> DFQSESYKDAYSRINAIVIEGEQEAFDNYNRLAEMLPDQRDELHKLAKMEQRHMKGFMACGKNLSVTPDMGFAQKFFERLHENFKAAAAEGKVVTCLLIQSLIIECFAIAAYNIYIPVADAFARKITEGVVRDEYLHRNFGEEWLKANFDASKAELEEANRQNLPLVWLMLNEVADDARELG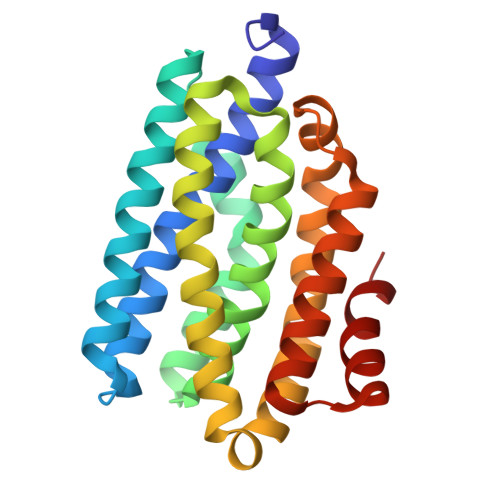MERESLVEDFMIAYGEALENIGFTTREIMRMSAYGLAAV> GSHMDNQCTVQVRLELGHRAQLRKKPTTEGFTHDWMVFVRGPEQCDI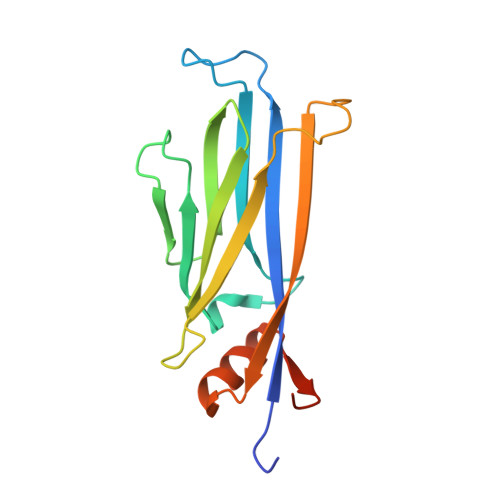QHFVEKVVFWLHDSFPKPRRVCKEPPYKVEESGYAGFIMPIEVHFKNKEEPRKVCFTYDLFLNLEGNPPVNHLRHLRCEKLTFNNPTTEFRYKLLRAGGVMVMPEGAHHHHHH> CNPQQTRRKQQYASIIGKQG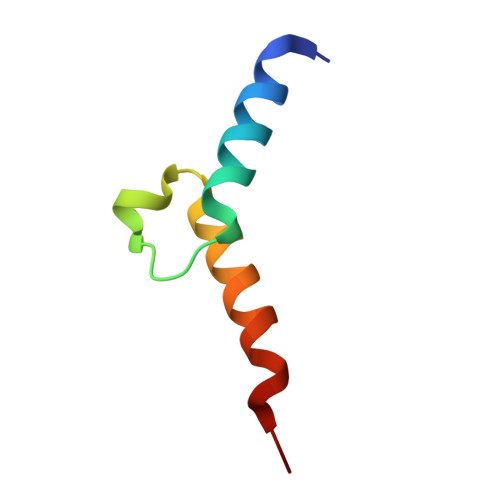LSKKQCGIFWDYYKRKCKKRRSTKKFI> SGTISSASFHPQQFQYTLDNNVLTLEQRKFYEENGFLVIKNLVPDADIQRFRNEFE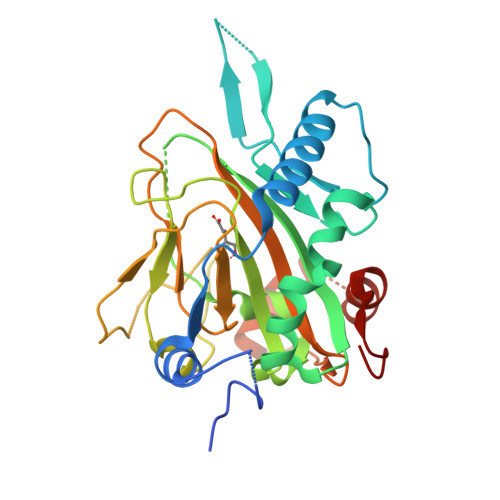KICRKEVKPLGLTVMRDVTISKSEYAPSEKMITKVQDFQEDKELFRYCTLPEILKYVECFTGPNIMAMHTMLINKPPDSGKKTSRHPLHQDLHYFPFRPSDLIVCAWTAMEHISRNNGCLVVLPGTHKGSLKPHDYPKWEGGVNKMFHGIQDYEENKARVHLVMEKGDTVFFHPLLIHGSGQNKTQGFRKAISCHFASADCHYIDVKGTSQENIEKEVVGIAHKFFGAENSVNLKDIWMFRARLVKGERTNL>[3x]GSRTAELQAEIDDTVGIMRDNINKVAERGERLTSIEDKADNLAVSAQGFKRGANRVRKAMW;>ALAEVQARHQELLKLEKSMAELTQLFNDMEELVIEQQENVDVIDKNVEDAQLDVEQGVGHTDKAVKSAR[3x];>[3x]GSIKFTKQSSVASTRNTLKMAQDAERA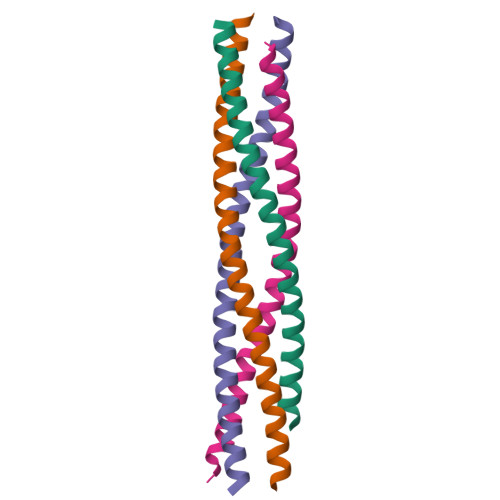GMNTLGMLGHQSEQLNNVEGNLDLMKVQNKVADEKVAELKKLQ;>GSEMELEIDRNLDQIQQVSNRLKKMALTTGKELDSQQKRLNNIEESTDDLDINLHMNTNRLAGI[3x]>HHHHHHSSGLVPRGSHMASMSKVGINGFGRIGRLVLRRLLEVKSNIDVVAINDLTSPKILAYLLKHDSNYGPFPWSVDFTEDSLIVDGKSIAVYAEKEAKNIPWKAKGAEIIVECTGFYTSAEKSQAHLDAGAKKVLISAPAGEMKTIVYNVNDDTLDGNDTIVSVASCTTNCLAPMAKALHDSFGIEVGTMTTIAAYTGTQSLVDGPRGKDLRASRAAAENIIPHTTGAAKAIGLVIPELSGKLKGHAQRVPVKTGSVTELVSILGKKVTAEEVNNALKQATTNNESFGYTDEEIVSSDIIGSHFGSVFDATQTEITAVGDLQLVKTVAWYDNEYGFVTQLIRTLEKFAKL[4x]

Glyceraldehyde-3-phosphate dehydrogenase (GAPDH) is a highly conserved enzyme involved in the ubiquitous process of glycolysis and presents a loop (residues 208–215 of Escherichia coli GAPDH) in two alternative conformations (I and II). In the presence of inorganic phosphate (Pi), GAPDH catalyzes the conversion of D-glyceraldehyde-3-phosphate (G3P) to 1,3-diphosphoglycerate (BPG), accompanying the reduction of NAD+ to NADH. All the structures reported in this paper have four subunits: O, P, Q, and R. Each subunit contained two domains: the C-terminal catalytic domain and the N-terminal NAD+-binding domain. Two anion recognition sites, “Ps” and “Pi”, bind the C3 phosphate of G3P and inorganic phosphate, respectively.

The enzymatic activity of wild-type EcGAPDH1 was 3.84 × 104 times higher than that of C150S and 8.13 × 103 times higher than that of H177A. Superimposing the backbone atoms from the structures of C150S.NAD, C150A.NAD, H177A.NAD, and C150AH177A.NAD on WT.NAD, it was found that the RMSDs were 0.134 (1266), 0.182 (1135 atoms), 0.135 (1247 atoms), and 0.122 Å (1219 atoms), respectively. This indicated that mutants have a very similar structure to the wild type.>[2x]MAPTFQTALFFTIISLSFAAPNAKQVRWCAISDLEQKKCNDLVGSCNVPDITLVCVLRSSTEDCMTAIKDGQADAMFLDSGEVYEASKDPYNLKPIIAEPYSSNRDLQKCLKERQQALAKKMIGHYIPQCDEKGNYQPQQCHGSTGHCWCVNAMGEKISGTNTPPGQTRATCERHELPKCLKERQVALGGDEKVLGRFVPQCDEKGNYEPQQFHGSTGYSWCVNAIGEEIAGTKTPPGKIPATCQKHDLVTTCHYAVAMVKKSSAFQFNQLKGKRSCHSGVSKTDGWKALVTVLVEKKLLSWDGPAKESIQRAMSKFFSVSCIPGATQTNLCKQCKGEEGKNCKNSHDEPYYGNYGAFRCLKEDMGDVAFLRSTALSDEHSEVYELLCPDNTRKPLNKYKECNLGTVPAGTVVTRKISDKTEDINNFLMEAQKRQCKLFSSAHGKDLMFDDSTLQLALLSSEVDAFLYLGVKLFHAMKALTGDAHLPSKNKVRWCTINKLEKM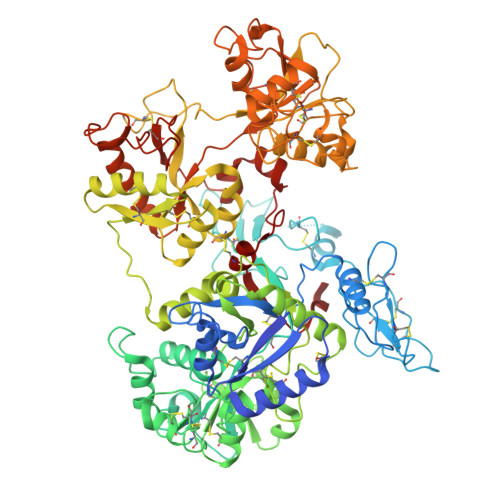KCDDWSAVSGGAIACTEASCPKGCVKQILKGEADAVKLEVQYMYEALMCGLLPAVEEYHNKDDFGPCKTPGSPATDFGTLRAVALVKKSNKDINWNNIKGKKSCHTGVGDIAGWVIPVSLIRRQNDNSDIDSFFGESCAPGSDTKSNLCKLCIGDPKNSAANTKCSLSDKEAYYGNQGAFRCLVEKGDVAFVPHTVVFENTDGKNPAVWAKNLKSEDFELLCLDGSRAPVSNYKSCKLSGIPPPAIVTREESISDVVRIVANQQSLYGRKGFEKDMFQLFSSNKGNNLLFNDNTQCLITFDRQPKDIMEDYFGKPYYTTVYGASRSAMSSELISACTIKHCSNSLEVL> MSKEIPTPYMWSYQPQMGLAAGASQDYSSRMNWLSAGPHMIGRVNGIRATRNQILLEQAALTSTPRSQLNPPNWPAAQVYQENPAPTTVLLPRDAEAEVQMTNSGAQLAGGSRHVRFRGRSSPYSPGPIKRLIIRGRGIQLNDEVVSSLTGLRPDGVFQLGGAGRSSFTPRQAYLTLQSSSSQPRSGGIGTLQFVEEFV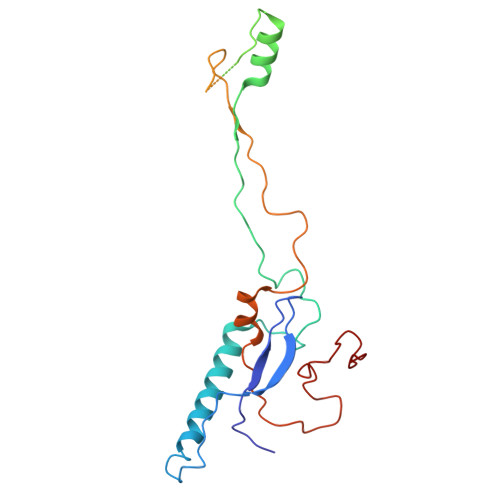PSVYFNPFSGAPGLYPDDFIPNYDAVSESVDGYD Arabinoxylan arabinofuranohydrolases belonging to the GH62 family specifically remove α-1,2- or α-1,3- linked L-arabinofuranose decorations from xylan (Kellett et al., 1990). For the GH62 enzymes of S. thermophilum sequences of Abf62A/Abf62B belongs to subfamily GH62_2, while Abf62C is a member of the GH62_1 subfamily. Abf62A and Abf62C are both active against these substrates but have no detectable activity against CM-linear 1,5-α-L-arabinan, which contains exclusively non-terminal 1,5-α-L-arabinofuranose linkages, indicating that these enzymes lack endo-arabinanase activity. 1HNMR spectroscopy showed that both Abf62C and Abf62A are active against both α-1,2 and α-1,3 L-arabinofuranosyl linkages in wheat arabinoxylan.

The crystal structures of Abf62C in apo form and in complex with xylotriose were determined to 1.23 Å and 1.48 Å resolutions respectively. The Abf62C apo structure was determined using a selenomethionine substituted protein crystal by the single wavelength anomalous diffraction (SAD) method, and it was then used as a search model to determine the structure of the Abf62C-xylotriose complex by the molecular replacement method. The Abf62C apo structure contains one polypeptide chain (residues 30 to 350) in the asymmetric unit. In addition, five phosphate ions and one glycerol molecule were modelled. Each ‘blade’ in this fold consists of either four (‘blade’ I, II, IV and III) or five (‘blade’ V) β-strands forming antiparallel β-sheets that are interconnected through loops of variable lengths to form a funnel-like structure that encircles the central cavity, which houses the active site. A comparative sequence analysis was undertaken to detect sequence conservation among various members of the two GH62 subfamilies, including structurally characterized representatives from the basidiomycete Ustilago maydis (UmAbf62A) and the ascomycete Podospora anserina (Siguier et al., 2014) points to three completely conserved residues Asp55, Asp171 and Glu230 as the catalytic triad of Abf62C. Interestingly, one of the phosphate molecules present in the Abf62C apo structure is bound in the active site cavity forming a network of hydrogen bonds with side chains of active site residues (Lys54, Arg259, His303 and Gln328) including that of the catalytic Glu230, thus suggesting the probable position of arabinose binding. Surprisingly, despite significant sequence similarity between PaAbf62C and Abf62C enzymes (64% identity) and also the conserved calcium binding residue (H285 in PaAbf62C and His303 in Abf62C), the Abf62C structure does not harbour a calcium ion in its active site. This Abf62C feature is in line with the functional data presented above, which shows that Abf62C activity is not significantly affected by the presence of Ca2+ or chelating agents, suggesting structural and functional independence from divalent metal ion binding.

> MGSSHHHHHHSSGRENLYFQGSSWKWVSTGPLVFPKNDERNIAGIKDPTAVLINGTYHVFASTAKSEGYNMVYFNFTDFAEANNAPFYYLDQAPLGYGYRAAPQVFYFEPHKLWYLVYQNGNAAYSTNPDINDPSKWTAPEVFYPNGMPKIIADNIGNGYWVDMWVVCDDEEDPNKALCHLFSSDDNGHLYRSQTTLAQFPRGMSEPEIVLQDTQNIYALWEAACIYRIKGAEGTQKYLLLVEAIGQEGHRYFRSWTSDRIDGQWIPLADTEANPWAGEANVVFEGQKWTKSISHGEVIRTLTDQTLTLDLSEPIQFLYQGVDPNAQTEYNALPWRLGLITQ> TTTTTTTTTGCAATAAAGCCTCAGAGAATTAGCAAAATTAATTTTTTTTT;> TTTTTTTTTAATCATACAGGCAAGGGCATTAACATCCAATATTTTTTTTT;> TTTTTTTTTCAATTCTACTAATAGTGCTGAAAAGGTGGCATTTTTTTTTT;> TTTTTTTTTCAGCTGTGGAGTAGATTAAGATGGCAGGTATGTTTTTTTTT;> TTTTTTTTTTGGGGGCACATGAGTGAGTTTTGGTACCAGGCTTTTTTTTT;> TTTTTTTTTACGAGTAGATTTAGAGTCAACATGTTCTGCGATTTTTTTTT;> TTTTTTTTTTCCCAATTTTAAATATCCATATAACAGTTGATTTTTTTTTT;> TTTTTTTTTCTAATTTTAAGACAAGATGATACAGTGTCTAGTTTTTTTTT;> TTTTTTTTTGCGGGCGCTAGGGCGCGAAGAAAGCGAAAGGATTTTTTTTT;> TTTTTTTTTCACCAGAACCCCAGCTGGCTTGTTGTGGAAGTTTTTTTTTT;> TGTCTAATGTATGGACAGTGGATAAACACGCGCCCTGTAGCGGCGCATTAAGCGCGGCGGGTGTGGTGGTTACGCGCAGCGTGACCGCTACACTTGCCAGCGCCCTAGCGCCCGCTCCTTTCGCTTTCTTCCCTTCCTTTCTCGCCACGTTCGCCGGCTTTCCCCGTCAAGCTCTAAATCGGGGGCTCCCTTTAGGGTTCCGATTTAGTGCTTTACGGCACCTCGACCCCAAAAAACTTGATTTGGGTGATGGTTCACGTAGTGGGCCATCGCCCTGATAGACGGTTTTTCGCCCTTTGACGTTGGAGTCCACGTTCTTTAATAGTGGACTCTTGTTCCAAACTGGAACAACACTCAACCCTATCTCGGGCTATTCTTTTGATTTATAAGGGATTTTGCCGATTTCGGGTAGAATTGGTAAAGAGAGTCGTGTAAAATATCGAGTTCGCACATCTTGTTGTCTGATTATTGATTTTTGGCGAAACCATTTGATCATATGACAAGATGTGTATCTACCTTAACTTAATGATTTTGATAAAAATCATTATAATGCCAGGGTCAGTGAGATGTAACACTACAGACCTCAGCTTCCTCTACTTTGCCTGGCATAGCCTACTGCACCATCCTTTTCAATGGAAGTAATTTGTCCCCCATGGGTTACACCCCCACCTAGACTACTTAAGAAGGTGCTATTGCTCCTGATTTCCAATGTTTGAATCTCCCTCCCACCATACCAGGCATAAAGGCTGTCACTCCCCAATACTAAGTGGCCCCAAGTTCACCACAATACAGCCAAGTGCATTGTTATCACATTCAGTCAAAGAATTTTCATTGGCAACAGTCCTCTCCAATCTGCCTATTCACTGTCCCTACATCAGGTGATAGTCCAGTTGTCAGACATGTGATCCCTGTTTGGGGACCCACAAGGCCTATCCAACCCATTGCTTTTAAAAGAGCTGGGGTTCTGGTGACTTCCACAACAAGCCCATCTGCTCTTAGTACAGCTTGTCTTAAAATTAGCTAGACACTGTATCATACCCCCTCCACTGCCCTATGATAAGGACAGCAGAGGGTTAGATTTACTTATCTGCACTCATGTGCCCCCAGCCTGGTACCAAAACTGATAATCTACTCCACAGCTGCATACCTGCCATCTTAGCCAAACCACACCAATCCAATTGCTGGGTCTCATATCATCTCTGAAGAAGTGATTACCTCATTACATGCTTGCTTGATATACCCACTTTCCTTATGAGGCACACCCATACTGAGGTAGCTATTTTACTATTGACTGGGTAAGCCAGTACAAAATAATCATAGGTGCACAGTCTGGACATGGGAACCCCTCTTCCTACTCACCTCTCTCAGAGGCAATGCCCCTTCATTAACCATGCACCCTAGGCCTTGGTACAAGTTGCCAACCTGCAGAGAACCAGTTAGCTGAAAGGCCAGGTTCTTCTTGATCTTGGTGCTTAGGGCAAACTTTTGGGATAGGCAAAAACAAGTCCTTTACACACCTCCAGTCTACAGTTCCATCAAAGTGGAACTTGGAATGTTATAAACTGCATCTATACTGTACTGCTAGTAGGCTTGTTTAATGCTTTCAACTCCTAGAGAATCACTTCAATCCTACCAACCAATAGTTCCCCATCACACAGATGGCTAAAGACCCTACCTCCCCTAAAGCCCTACTTCACACTGCAGGGACCTCCTAAGGGTCTTGGACCCTCCTCACTTGTTACTAGGCTATCATTCTACTGGTGCAGATACAGATTTTAGGTACCTGTCCTTGATGCACTTAGCTTTAACATGTCACATGCCAATGAAAATAGCAGCCACAGGGGGATATTCTAGGAGCAACATGGAGACTGTCTGCTACAACCACCAAACAGCTCATCCTCTGCATGAATACTTACTCTAGACCCCTGCATTCACCTTCCATGATTAATCACCAACTGAGTCTTGCAAAACCCAATTATGGTTATAGACAGACTGGCCCATGTTACCACTTAAACTCCATCTAGTCTGCAGTGTTCTGACCTATGCCTGAGGGTCCAGATAACCACTCTTCACTAAGCCCCCTGGAAGACAGTTAAGTCTATCTATCAGCCTCACATCCATCCCATTCTCTCTTTGAGATCTTATCAGGACTGATTGTATGTGAACAATATACTCCCAGGCTGGCCATTAGAGATTGGTTAGTGGTTGGCTGGACCAACACCCTTAAGCAACTAATAAGACCATGTGGGGTGTCCAGGCCTCATAAATCCTGAGCCTCTCAATCTTCCAGTGGCTCACCATTCCCATCCACACAACCTATTGGAACCATCAGAGTCATCACCTATATAGGGTGAAGTAGAGCTCCACCACCCCATAACTATACAGTGCACCTGGCCTCTGAGACTTGCTGTGATAACACAAACCCCAGGGCCAAATTGGGAAGATGCAATGACATTCCATTACTTCTCCAGGACAACATTTATTTGTTGCTGACTCCAGACTTAACAAGGAGTATTTGAGGCCACTGTTGGGGCCCTAACCCACCCAGCTCTTGACAGCTAATCTTAACCTCAAGGATTGACCATTGGGGGAGTCAACCAGCTTTGGCCCTGCTCAAGCAAACAATCCCCAGATGACCTGCTGGCAGGCACCCCTAGAAATATTGTGGGTTGCACTATTTCTTGCTCAGATGCTTCCCACTATAGCCCCACTCCAACTAGTACCACATCATTTTATGGATCAATCACAAAGGAGCCCCTATAGGCTGATTCTGTGTTTCAAAAAGTGAAGCCTATGTGCTCCATTGAGTCAGTAAATTAACACCACTAGAAGTTATCCAGCTAGTCAAGGGTTTTCCATATGTCCCAAGGTACTAGCTACAGCACTTGAATATGGTCTACTATGAGTGGGACTATTAATGTCATCTTTCTGTATAGCTGCCCCATTTAAAGCATATATGAAGTGCTAACATTGTGTTGGATCTTTATGCCACCAGATCCCCCTTACAGTATTCTCACCCAAATGGGATGAGAGTTGTATTAAGGCTAGTTAATCCCTAAGTCCATACATAGGACCACAGTAGCTTGGCTATGCTCACAATTTGCCATGTATATCAGTCCCAGAGGTATGCAAGACATTGCCCACATTTCAGAATGGTCCTGTCTTGTGGTTCCTTGCCTTTTGCACATTACCCTTGGCCTTCTACATAATGTGAGTCCTGGCTGCAATCTATGTATTGAAAGTAGGTAACCCTTCTCATTGTCAAGAACATCTGTTCCTAGCCACCCTGACCCTGCCTCCCTGAAGCTGCTCCCATAGGCCCACTGATCTCACTGCTTCTAATTGCATCCCTTGACTCTCTATCCCCTGAGAATTCCTGCTTGTGCAGCCTTGTGAGCCACTACCCAGTCAGGGTGTTAAGCCTTACCATGACCAGGTGCCCTCTATGACTAGCCCAAGACTCACAGACAGGATAGCCAGCTGTACCCCACACTCCTCTTGCCCTGGGCACTCTCATCAGTACCCTCAATAACCTAGCTGTCCACTCACTATCCTCAGACCAATTCTCCTTCTGCCAAAGGTCCAACATAGAGGACTCATCTGGGCTCAGGCAACTCAGGGCATATGGGACCATAGCTCAACTACAATAAAACCAGGGGCCACATAAGCTAGCAATCAGTGGGTGTAAGTGTCTGGGTGCATCAGCTGGTAAGACTGCCAGATTCTATGCAGGCCAATCATGAACCTACTAGTCCCTCATGGTCACTTTGTTCATCTAACAGATAGTTGCTTCAAACTCAAGACCTTACTAACCTTAGTCACTGGTTCTACCAGCCCAGGAATCCTCCTTGGGCTAGCCTCCAAGAAGCTTCAGACTCCTTAATACCAAGCAGCAGGAACAGTTTCAGCACCAAGAGGTGAGAACTGCTGTTAGCATCACTGACTTACAATCTCATGATAGCTAAGCATTCTTAGAACTCTTATATAACTCCCTATTACCAGAGACAGCCCTCAGGATTACTGATGGACCTTCTTCAAGTCTTTTCTAGCACAGGACCTACAGGGAGAGGGAAAGTCAGCTCCTATGGGGAATACAAGAGTTAGTCTTCAGTTTGTGGCTGAGGCTTCTTTGTGCTGGTTGCCTCTAAGACAAATTATTCTGGAATCTAATCAAGTTTACAAGGTCAGCATTATGACCCAGGTCAATAGCTTCTGGGAGGCTCTTCTAGTTTCCACCTTTGTACCAGTATCCTATTTAAGATAGGTCATGCATAGGGCTCTACACAATGAGTTCAGAGCCTTTGCAGCTTAAGGAAATCTCTCCTCCATAAAAGTTCTGCTTTGATGTCAATTCCCCTTGTACTTCCTGTGACTGCAACACAGTTGGACTGGTATTCCTCAACATCAACAATTAGTAAAAGCAATGGTTGTGACCAAGGAATGAGACCAGCAATTAATTGACATAGTTTAACTGTCAAACACTGAGAGATGGAGCCTGCAAGTGGGGCTTATCCCACAGAGTACTGTTTTCTGAGGAGCTGAGTTAACAGGTGGAGAAAATCCCAAAGATACTCTCCCAATGGCCAGTCCAAGCTTGAAGTCAATGCAACCTCTAGTAATAGGTAGAGGCTGCCACAAATGATGCCTACAAAGAGTAAACTTCTATATGTGGTAATGGCATCCAAGTAAAGGGCTAATGCAGAACAGAGCTTTTGTTAATGGGCAAGCTACTACTAAACCCTCTGGAGCATGTGTTAGTAGATACCTTCAACCTTGGAGCTCACTCAGAAAAAGCCTGAACCCAGAATTAAAACATCCTGGTGTACTCTGGCACCAGTGACACCATGGCTTTTTCAGGCCCCTGTGCCTGTTGCATGCAAACCTAAGAGTCTAAAGGTAATCTGTCAGCCAGGAGAGTGGTCTCCATGCCTCAGTGTGTAGGTGGGCAGTCATTCCTATACCATATAAAATGGAGTACATCTACAAGCACTGGACTACCTAGGTTTCCTGGATAGTAACTCTAACCAGACACACATGGCCTGGAGTGGAGTTACCCAACAGAACCCTGTCATATTTCCTAATCCACTAAAGTCTGTTACATACAGGCAGTTTTTGCTCTCTGCTGCCTGCCCAGCAGCTATGGTGATCAACTGGCTAGAATGACTTGTGTACCTACCCTAATTTTAATTTCACTCTGACATGCAGTTCAACAGGCTACCCCTTTTTATTGGTGGCTACATTTGGCTTAATTCTAACTGGTCAGAGATAAAGCTCAGCAGTGATATGAGCCCTTAGGAAAATTCCAGAGCACACACTAGCAGATGTTTTATCATGGAATATTATCAATGTAGCTCTGGGGGTAACTTTGAAAAGCTGTTCACTTACCTTTCCAGGGATAACTTGCATTTAGACATACTAGATTATCTTACATTCTGATATCACTAGTGTCCTGAAACAGGGCTTCATCATAATCCTTGTCACCTGTTAAACCTTTTATATGCCCTTGCTAGGGCCCAACTCTGTCTCCTGTAAAGTTAAAGTGCCTTCAGGAAGTTGGTGAGTAGACCTGAATAATTCATACTTTATCTCCTACACCAGGATGACTCAGTAGGACATCTCAGTCTCTAATACTCATACAAATACACTCTATTAGGGGCTGGGACACCTGATCCAGAAACAAAGTTTCTTAAGTACCTCTGTACAATTGAAGATAATGGTACTCAATGATATTTTGTGATTCAAATTTACAGAGAGCAGTAATGTTCCCAGTTTATCCTTAGATAGAGCAAAAGATTAAAGAACCTGGTTAATATTTAGGATCTGATGATCCTGCACACTTCTGAATGCCTTGAAATTCTTGTCCATTCAATACCCTGGTCTTAGGCCATATCCTGTTCTAGAACACTTATGCACAATCAATATGCATGGGCTGTGTGAGGGCTGCTATCTGTAGGCACTAATGGATTTGTAAGCTGGCTCTGTTTCTCTTACTTTCAGTATACCTATCAAGGTTTTGGTGTTGAAACCTGACTGACCACTGGCAAAGGGTGGGAAACTTAGGTTCCCTAGTATGCTAGCTTAGCAACCATAAGGTCTATTGTCTCAAATCAAAATCTAGGGGAACATGATCTGGATGCCCATATTCAAGCCAACAAATCTTGAACTGGGATTCCAAGGGCCTAACAACTATTCCACTTGGCACTTTAGCAGGCTCATTCATGCTCTGATCAGTTGCAATTTATGAAACTGTAGTCTCAGGTCCTAGGAATTATAGGTTGTACACTGGGCCTCCTGGGAATTGTTTGCTACTTGACCTCTTTCATGTACATGTTGATGGGGTAGTACTAATTAAGAGCCATAGTCATAAGTAGTTGGGCATGCTGAATCATCCAGTAGAAGGCTCCAGCATGAGGTGGCATTGATGAACAGCCTAAGCTTATTGCAAGCATGGCACATAGCACCTAACTTCATGACTGTTATTCATTTACCTGAGTATAGGATTTCATATAGATCCAAATAGGAACTAAGGTTCATAGTAGCCATCATGTTCAAAGCTATAACAAACATTAAATATATCCATGTCCTAAATGCATTAGGTGAACCAAGTCACAGGTACAGAAAGGGGATGCAGCACAAAAATTGATACTTGTAGAAAGAGGATTCAGATATATTGAGCTGTGCTACCATTAATAAAGATGGGTCCCATGAAGAGCATCTTCTGTTGTTAGGTCTGACTATGGCAGCAAATCCAGGTAAGGCAAGGACTAGTTCTCAAGTGACCTTTAAGTTGACTTTTAGCCTGTATTTCAAGGCTTAGAGGGCACAACTGTGTCTATAAATTGCCTAATGAATCCATAGACTTTACCAATGCTGTCTAGATATGCTTAAAGGAAGAGTGTTGTAGTGTATGAACTTTCTATTTGCTGCTGAGATATTAGTTGTGGATCCTAGTTGAATTTCTAAGTTAGGCAGGTATCTGGCTTGCAGGATCCATTTCTGCAAAGTAAGAGGGGGTCATTGCAGACCCATGCTATGTCTGTGAAAGATCTGTGCATATCTAGAGGTTAGGACTTCAGCTACCTGGGTTTGCATAAGAATAAGCAGACTAAAAGGCATGACAGAAGACTTCTTATGGGTAGCAGTCTTATTTTTAGAGTTCTTGGGAGATCAGATCTAAGGAGATTCACAAGAAACTAGAGTAGCATTGGAGATGAGTAACATATACACATATTACTACATGGTTTACTGCCTTAAATGTGGCCTAGGGTATTATGCTGGAGAGCTAGGTGTCAGTTCTAAAAAGGATAAGTCATGGGGGCCTTTCACAGCAAGTTACAAACTATGTTTAGTATCAGAACTTATTAAACATAACAGTAACCAAAGCCATGGTATGATGTACTATCTTTTTGTAGCACTAGGATACTATATTAACTACTCTTTAGTTTTGTCATGAGAAGTACACCTTATAGCATAGATTGAATGGGTGGATGTCTCTGTGGAGGTGTGTGCTTGGATTAGATGGTGTGAATAGAAAACTAAATACTGGATTGGACAAGTGTT;> TTAAGCTCTAAGCCATCCGCAAAAATGACCTCTTATCAAAAGGAGCAATTAAAGGTACTCTCTAATCCTGACCTGTTGGAGTTTGCTTCCGGTCTGGTTCGCTTTGAAGCTCGAATTAAAACGCGATATTTGAAGTCTTTCGGGCTTCCTCTTAATCTTTTTGATGCAATCCGCTTTGCTTCTGACTATAATAGTCAGGGTAAAGACCTGATTTTTGATTTATGGTCATTCTCGTTTTCTGAACTGTTTAAAGCATTTGAGGGGGATTCAATGAATATTTATGACGATTCCGCAGTATTGGACGCTATCCAGTCTAAACATTTTACTATTACCCCCTCTGGCAAAACTTCTTTTGCAAAAGCCTCTCGCTATTTTGGTTTTTATCGTCGTCTGGTAAACGAGGGTTATGATAGTGTTGCTCTTACTATGCCTCGTAATTCCTTTTGGCGTTATGTATCTGCATTAGTTGAATGTGGTATTCCTAAATCTCAACTGATGAATCTTTCTACCTGTAATAATGTTGTTCCGTTAGTTCGTTTTATTAACGTAGATTTTTCTTCCCAACGTCCTGACTGGTATAATGAGCCAGTTCTTAAAATCGCATAAGGTAATTCACAATGATTAAAGTTGAAATTAAACCATCTCAAGCCCAATTTACTACTCGTTCTGGTGTTTCTCGTCAGGGCAAGCCTTATTCACTGAATGAGCAGCTTTGTTACGTTGATTTGGGTAATGAATATCCGGTTCTTGTCAAGATTACTCTTGATGAAGGTCAGCCAGCCTATGCGCCTGGTCTGTACACCGTTCATCTGTCCTCTTTCAAAGTTGGTCAGTTCGGTTCCCTTATGATTGACCGTCTGCGCCTCGTTCCGGCTAAGTAACATGGAGCAGGTCGCGGATTTCGACACAATTTATCAGGCGATGATACAAATCTCCGTTGTACTTTGTTTCGCGCTTGGTATAATCGCTGGGGGTCAAAGATGAGTGTTTTAGTGTATTCTTTTGCCTCTTTCGTTTTAGGTTGGTGCCTTCGTAGTGGCATTACGTATTTTACCCGTTTAATGGAAACTTCCTCATGAAAAAGTCTTTAGTCCTCAAAGCCTCTGTAGCCGTTGCTACCCTCGTTCCGATGCTGTCTTTCGCTGCTGAGGGTGACGATCCCGCAAAAGCGGCCTTTAACTCCCTGCAAGCCTCAGCGACCGAATATATCGGTTATGCGTGGGCGATGGTTGTTGTCATTGTCGGCGCAACTATCGGTATCAAGCTGTTTAAGAAATTCACCTCGAAAGCAAGCTGATAAACCGATACAATTAAAGGCTCCTTTTGGAGCCTTTTTTTTGGAGATTTTCAACGTGAAAAAATTATTATTCGCAATTCCTTTAGTTGTTCCTTTCTATTCTCACTCCGCTGAAACTGTTGAAAGTTGTTTAGCAAAATCCCATACAGAAAATTCATTTACTAACGTCTGGAAAGACGACAAAACTTTAGATCGTTACGCTAACTATGAGGGCTGTCTGTGGAATGCTACAGGCGTTGTAGTTTGTACTGGTGACGAAACTCAGTGTTACGGTACATGGGTTCCTATTGGGCTTGCTATCCCTGAAAATGAGGGTGGTGGCTCTGAGGGTGGCGGTTCTGAGGGTGGCGGTTCTGAGGGTGGCGGTACTAAACCTCCTGAGTACGGTGATACACCTATTCCGGGCTATACTTATATCAACCCTCTCGACGGCACTTATCCGCCTGGTACTGAGCAAAACCCCGCTAATCCTAATCCTTCTCTTGAGGAGTCTCAGCCTCTTAATACTTTCATGTTTCAGAATAATAGGTTCCGAAATAGGCAGGGGGCATTAACTGTTTATACGGGCACTGTTACTCAAGGCACTGACCCCGTTAAAACTTATTACCAGTACACTCCTGTATCATCAAAAGCCATGTATGACGCTTACTGGAACGGTAAATTCAGAGACTGCGCTTTCCATTCTGGCTTTAATGAGGATTTATTTGTTTGTGAATATCAAGGCCAATCGTCTGACCTGCCTCAACCTCCTGTCAATGCTGGCGGCGGCTCTGGTGGTGGTTCTGGTGGCGGCTCTGAGGGTGGTGGCTCTGAGGGTGGCGGTTCTGAGGGTGGCGGCTCTGAGGGAGGCGGTTCCGGTGGTGGCTCTGGTTCCGGTGATTTTGATTATGAAAAGATGGCAAACGCTAATAAGGGGGCTATGACCGAAAATGCCGATGAAAACGCGCTACAGTCTGACGCTAAAGGCAAACTTGATTCTGTCGCTACTGATTACGGTGCTGCTATCGATGGTTTCATTGGTGACGTTTCCGGCCTTGCTAATGGTAATGGTGCTACTGGTGATTTTGCTGGCTCTAATTCCCAAATGGCTCAAGTCGGTGACGGTGATAATTCACCTTTAATGAATAATTTCCGTCAATATTTACCTTCCCTCCCTCAATCGGTTGAATGTCGCCCTTTTGTCTTTGGCGCTGGTAAACCATATGAATTTTCTATTGATTGTGACAAAATAAACTTATTCCGTGGTGTCTTTGCGTTTCTTTTATATGTTGCCACCTTTATGTATGTATTTTCTACGTTTGCTAACATACTGCGTAATAAGGAGTCTTAATCATGCCAGTTCTTTTGGGTATTCCGTTATTATTGCGTTTCCTCGGTTTCCTTCTGGTAACTTTGTTCGGCTATCTGCTTACTTTTCTTAAAAAGGGCTTCGGTAAGATAGCTATTGCTATTTCATTGTTTCTTGCTCTTATTATTGGGCTTAACTCAATTCTTGTGGGTTATCTCTCTGATATTAGCGCTCAATTACCCTCTGACTTTGTTCAGGGTGTTCAGTTAATTCTCCCGTCTAATGCGCTTCCCTGTTTTTATGTTATTCTCTCTGTAAAGGCTGCTATTTTCATTTTTGACGTTAAACAAAAAATCGTTTCTTATTTGGATTGGGATAAATAATATGGCTGTTTATTTTGTAACTGGCAAATTAGGCTCTGGAAAGACGCTCGTTAGCGTTGGTAAGATTCAGGATAAAATTGTAGCTGGGTGCAAAATAGCAACTAATCTTGATTTAAGGCTTCAAAACCTCCCGCAAGTCGGGAGGTTCGCTAAAACGCCTCGCGTTCTTAGAATACCGGATAAGCCTTCTATATCTGATTTGCTTGCTATTGGGCGCGGTAATGATTCCTACGATGAAAATAAAAACGGCTTGCTTGTTCTCGATGAGTGCGGTACTTGGTTTAATACCCGTTCTTGGAATGATAAGGAAAGACAGCCGATTATTGATTGGTTTCTACATGCTCGTAAATTAGGATGGGATATTATTTTTCTTGTTCAGGACTTATCTATTGTTGATAAACAGGCGCGTTCTGCATTAGCTGAACATGTTGTTTATTGTCGTCGTCTGGACAGAATTACTTTACCTTTTGTCGGTACTTTATATTCTCTTATTACTGGCTCGAAAATGCCTCTGCCTAAATTACATGTTGGCGTTGTTAAATATGGCGATTCTCAATTAAGCCCTACTGTTGAGCGTTGGCTTTATACTGGTAAGAATTTGTATAACGCATATGATACTAAACAGGCTTTTTCTAGTAATTATGATTCCGGTGTTTATTCTTATTTAACGCCTTATTTATCACACGGTCGGTATTTCAAACCATTAAATTTAGGTCAGAAGATGAAATTAACTAAAATATATTTGAAAAAGTTTTCTCGCGTTCTTTGTCTTGCGATTGGATTTGCATCAGCATTTACATATAGTTATATAACCCAACCTAAGCCGGAGGTTAAAAAGGTAGTCTCTCAGACCTATGATTTTGATAAATTCACTATTGACTCTTCTCAGCGTCTTAATCTAAGCTATCGCTATGTTTTCAAGGATTCTAAGGGAAAATTAATTAATAGCGACGATTTACAGAAGCAAGGTTATTCACTCACATATATTGATTTATGTACTGTTTCCATTAAAAAAGGTAATTCAAATGAAATTGTTAAATGTAATTAATTTTGTTTTCTTGATGTTTGTTTCATCATCTTCTTTTGCTCAGGTAATTGAAATGAATAATTCGCCTCTGCGCGATTTTGTAACTTGGTATTCAAAGCAATCAGGCGAATCCGTTATTGTTTCTCCCGATGTAAAAGGTACTGTTACTGTATATTCATCTGACGTTAAACCTGAAAATCTACGCAATTTCTTTATTTCTGTTTTACGTGCAAATAATTTTGATATGGTAGGTTCTAACCCTTCCATTATTCAGAAGTATAATCCAAACAATCAGGATTATATTGATGAATTGCCATCATCTGATAATCAGGAATATGATGATAATTCCGCTCCTTCTGGTGGTTTCTTTGTTCCGCAAAATGATAATGTTACTCAAACTTTTAAAATTAATAACGTTCGGGCAAAGGATTTAATACGAGTTGTCGAATTGTTTGTAAAGTCTAATACTTCTAAATCCTCAAATGTATTATCTATTGACGGCTCTAATCTATTAGTTGTTAGTGCTCCTAAAGATATTTTAGATAACCTTCCTCAATTCCTTTCAACTGTTGATTTGCCAACTGACCAGATATTGATTGAGGGTTTGATATTTGAGGTTCAGCAAGGTGATGCTTTAGATTTTTCATTTGCTGCTGGCTCTCAGCGTGGCACTGTTGCAGGCGGTGTTAATACTGACCGCCTCACCTCTGTTTTATCTTCTGCTGGTGGTTCGTTCGGTATTTTTAATGGCGATGTTTTAGGGCTATCAGTTCGCGCATTAAAGACTAATAGCCATTCAAAAATATTGTCTGTGCCACGTATTCTTACGCTTTCAGGTCAGAAGGGTTCTATCTCTGTTGGCCAGAATGTCCCTTTTATTACTGGTCGTGTGACTGGTGAATCTGCCAATGTAAATAATCCATTTCAGACGATTGAGCGTCAAAATGTAGGTATTTCCATGAGCGTTTTTCCTGTTGCAATGGCTGGCGGTAATATTGTTCTGGATATTACCAGCAAGGCCGATAGTTTGAGTTCTTCTACTCAGGCAAGTGATGTTATTACTAATCAAAGAAGTATTGCTACAACGGTTAATTTGCGTGATGGACAGACTCTTTTACTCGGTGGCCTCACTGATTATAAAAACACTTCTCAGGATTCTGGCGTACCGTTCCTGTCTAAAATCCCTTTAATCGGCCTCCTGTTTAGCTCCCGCTCTGATTCTAACGAGGAAAGCACGTTATACGTGCTCGTCAAAGCAACCATAGTACGCGCCCTGTAGCGGCGCATTAAGCGCGGCGGGTGTGGTGGTTACGCGCAGCGTGACCGCTACACTTGCCAGCGCCCTAGCGCCCGCTCCTTTCGCTTTCTTCCCTTCCTTTCTCGCCACGTTCGCCGGCTTTCCCCGTCAAGCTCTAAATCGGGGGCTCCCTTTAGGGTTCCGATTTAGTGCTTTACGGCACCTCGACCCCAAAAAACTTGATTTGGGTGATGGTTCACGTAGTGGGCCATCGCCCTGATAGACGGTTTTTCGCCCTTTGACGTTGGAGTCCACGTTCTTTAATAGTGGACTCTTGTTCCAAACTGGAACAACACTCAACCCTATCTCGGGCTATTCTTTTGATTTATAAGGGATTTTGCCGATTTCGGAACCACCATCAAACAGGATTTTCGCCTGCTGGGGCAAACCAGCGTGGACCGCTTGCTGCAACTCTCTCAGGGCCAGGCGGTGAAGGGCAATCAGCTGTTGCCCGTCTCACTGGTGAAAAGAAAAACCACCCTGGCGCCCAATACGCAAACCGCCTCTCCCCGCGCGTTGGCCGATTCATTAATGCAGCTGGCACGACAGGTTTCCCGACTGGAAAGCGGGCAGTGAGCGCAACGCAATTAATGTGAGTTAGCTCACTCATTAGGCACCCCAGGCTTTACACTTTATGCTTCCGGCTCGTATGTTGTGTGGAATTGTGAGCGGATAACAATTTCACACAGGAAACAGCTATGACCATGATTACGAATTCGAGCTCGGTACCCGGGGATCCTCCGTCTTTATCGAGGTAACAAGCACCACGTAGCTTAAGCCCTGTTTACTCATTACACCAACCAGGAGGTCAGAGTTCGGAGAAATGATTTATGTGAAATGCGTCAGCCGATTCAAGGCCCCTATATTCGTGCCCACCGACGAGTTGCTTACAGATGGCAGGGCCGCACTGTCGGTATCATAGAGTCACTCCAGGGCGAGCGTAAATAGATTAGAAGCGGGGTTATTTTGGCGGGACATTGTCATAAGGTTGACAATTCAGCACTAAGGACACTTAAGTCGTGCGCATGAATTCACAACCACTTAGAAGAACATCCACCCTGGCTTCTCCTGAGAAAGCTTGGCACTGGCCGTCGTTTTACAACGTCGTGACTGGGAAAACCCTGGCGTTACCCAACTTAATCGCCTTGCAGCACATCCCCCTTTCGCCAGCTGGCGTAATAGCGAAGAGGCCCGCACCGATCGCCCTTCCCAACAGTTGCGCAGCCTGAATGGCGAATGGCGCTTTGCCTGGTTTCCGGCACCAGAAGCGGTGCCGGAAAGCTGGCTGGAGTGCGATCTTCCTGAGGCCGATACTGTCGTCGTCCCCTCAAACTGGCAGATGCACGGTTACGATGCGCCCATCTACACCAACGTGACCTATCCCATTACGGTCAATCCGCCGTTTGTTCCCACGGAGAATCCGACGGGTTGTTACTCGCTCACATTTAATGTTGATGAAAGCTGGCTACAGGAAGGCCAGACGCGAATTATTTTTGATGGCGTTCCTATTGGTTAAAAAATGAGCTGATTTAACAAAAATTTAATGCGAATTTTAACAAAATATTAACGTTTACAATTTAAATATTTGCTTATACAATCTTCCTGTTTTTGGGGCTTTTCTGATTATCAACCGGGGTACATATGATTGACATGCTAGTTTTACGATTACCGTTCATCGATTCTCTTGTTTGCTCCAGACTCTCAGGCAATGACCTGATAGCCTTTGTAGATCTCTCAAAAATAGCTACCCTCTCCGGCATTAATTTATCAGCTAGAACGGTTGAATATCATATTGATGGTGATTTGACTGTCTCCGGCCTTTCTCACCCTTTTGAATCTTTACCTACACATTACTCAGGCATTGCATTTAAAATATATGAGGGTTCTAAAAATTTTTATCCTTGCGTTGAAATAAAGGCTTCTCCCGCAAAAGTATTACAGGGTCATAATGTTTTTGGTACAACCGATTTAGCTTTATGCTCTGAGGCTTTATTGCTTAATTTTGCTAATTCTTTGCCTTGCCTGTATGATTTATTGGATGTTAATGCTACTACTATTAGTAGAATTGATGCCACCTTTTCAGCTCGCGCCCCAAATGAAAATATAGCTAAACAGGTTATTGACCATTTGCGAAATGTATCTAATGGTCAAACTAAATCTACTCGTTCGCAGAATTGGGAATCAACTGTTATATGGAATGAAACTTCCAGACACCGTACTTTAGTTGCATATTTAAAACATGTTGAGCTACAGCATTATATTCAGCAAT;> TTTTTTTTTTGAGTGTTGTTCCAGTTAGCCCGAGATAGGGTTTTTTTTTT;> TTTTTTTTTGGGAAGAAAGCGAAAGCGTGGCGAGAAAGGAATTTTTTTTT;> TTTTTTTTTAAGTGTTTTTATAATCACGCCAGAATCCTGAGTTTTTTTTT;> TTTTTTTTTAATGGATTATTTACATACGCTCAATCGTCTGATTTTTTTTT;> TTTTTTTTTAATTTACTGACTCAATAACTTCTAGTGGTGTTTTTTTTTTT;> TTTTTTTTTCACAGAATCAGCCTGAGCTTCACTTTTTGAAATTTTTTTTT;> TTTTTTTTTGTGATTGATCCATATAGTATAGGGGCTCCTTTTTTTTTTTT;> TTTTTTTTTTAGTTGGAGTGGGGCAATAAATGATGTGGTACTTTTTTTTT;> TTTTTTTTTATCTGAGCAAGAAATTCTCTATAGTGGGAAGCTTTTTTTTT;> TTTTTTTTTATATTTCTAGGGGTGCGGTAGTGCAACCCACATTTTTTTTT;> TTTTTTTTTGATTGTTTGCTTGAGCCAGCAGGTCATCTGGGTTTTTTTTT;> TTTTTTTTTCCCCCAATGGTCAATCCCAAAGCTGGTTGACTTTTTTTTTT;> TTTTTTTTTTCAAGAGCTGGGTGGGAGGTTAAGATTAGCTGTTTTTTTTT;> TTTTTTTTTTCAAATACTCCTTGTTGGCCCCAACAGTGGCCTTTTTTTTT;> TTTTTTTTTGCCTTGAATCGGCTGAGGGCACGAATATAGGGTTTTTTTTT;> TTTTTTTTTTCTGTAAGCAACTCGTCAGTGCGGCCCTGCCATTTTTTTTT;> TTTTTTTTTGAGTGACTCTATGATAATTTACGCTCGCCCTGTTTTTTTTT;> TTTTTTTTTAATAACCCCGCTTCTAGACAATGTCCCGCCAATTTTTTTTT;> TTTTTTTTTTGCTGAATTGTCAACCATTTAAGTGTCCTTAGTTTTTTTTT;> TTTTTTTTTTTCATGCGCACGACAAATTAAGTGGTTGTGAATTTTTTTTT;> TTTTTTTTTGGTGGATGTTCTTCTTAATCAGGAGAAGCCAGTTTTTTTTT;> TTTTTTTTTAGTGCCAAGCTTTCGGTAGTAAAACGACGGCCTTTTTTTTT;> TTTTTTTTTCCAGTCACGACGTTGCCAACGCCAGGGTTTTCTTTTTTTTT;> TTTTTTTTTCAACCACTAACCAAACCTGGTGTTGGTCCAGCTTTTTTTTT;> TTTTTTTTTCCTGGGAGTATATTCATATCTCTAATGGCCAGTTTTTTTTT;> TTTTTTTTTAGTCCTGATAAGATTCCAGTTCACATACAATCTTTTTTTTT;> TTTTTTTTTGGGATGGATGTGAGGCTCCTCAAAGAGAGAATTTTTTTTTT;> TTTTTTTTTCTTCCAGGGGGCTTAGAGATAGACTTAACTGTTTTTTTTTT;> TTTTTTTTTCCTCAGGCATAGGTCAGAGTGGTTATCTGGACTTTTTTTTT;> TTTTTTTTTAGTTTAAGTGGTAACAACTGCAGACTAGATGGTTTTTTTTT;> TTTTTTTTTCATAATTGGGTTTTGCCCAGTCTGTCTATAACTTTTTTTTT;> TTTTTTTTTAGGTGAATGCAGGGGCGGTGATTAATCATGGATTTTTTTTT;> TTTTTTTTTTTCATGCAGAGGATATAAGTCTAGAGTAAGTATTTTTTTTT;> TTTTTTTTTTTGTAGCAGACAGTCAATGAGCTGTTTGGTGGTTTTTTTTT;> TTTTTTTTTTAGAATATCCCCCTGTCCCTCCATGTTGCTCCTTTTTTTTT;> TTTTTTTTTTGTGACATGTTAAAGCGCTATTTTCATTGGCATTTTTTTTT;> TTTTTTTTTACCTAAAATCTGTATCTGCATCAAGGACAGGTTTTTTTTTT;> TTTTTTTTTCTAGTAACAAGTGAGGCCAGTAGAATGATAGCTTTTTTTTT;> TTTTTTTTTAAAGCCCCAAAAACAGCCGGTTGATAATCAGATTTTTTTTT;> TTTTTTTTTGCATGTCAATCATATGGGTAATCGTAAAACTATTTTTTTTT;> TTTTTTTTTAAACAAGAGAATCGATCCTGAGAGTCTGGAGCTTTTTTTTT;> TTTTTTTTTCAAAGGCTATCAGGTCTTTTTTGAGAGATCTATTTTTTTTT;> TTTTTTTTTGAGAGGGTAGCTATGCAAATAAATTAATGCCGTTTTTTTTT;> TTTTTTTTTAACCGTTCTAGCTGGAAATCAATATGATATTCTTTTTTTTT;> TTTTTTTTTCAGTCAAATCACCAAATGAGAAAGGCCGGAGATTTTTTTTT;> TTTTTTTTTGCCTATCCCAAAAGAACCAAGGACTTGTTTTTTTTTTTTTT;> TTTTTTTTTCAAGATCAAGAAGACCTTTTTGCCCTAAGCACTTTTTTTTT;> TTTTTTTTTCTAACTGGTTCTCTGCGCACCTGGCCTTTCAGTTTTTTTTT;> TTTTTTTTTTGTAATACCCTGACTAGGAAACATTATGACCCTTTTTTTTT;> TTTTTTTTTATCGGTTGTACCAATAACGAGCATAAAGCTAATTTTTTTTT;> TTTTTTTTTATTGTTATCCGCTCACAACAATTCGAATCAATA;> AAAGAAATACATGGCTTTTTTGTATTTGGAGTTGGGTAGCCA;> GGGTCAGAAGGAGCAAGTTTGCAAGGAAGAGCATAAATATCT;> GTTTGAGGCAATTCCAACTCGTCATTAGACTTTACCGATTGG;> GAGAGTCAAGGGATGGGAGCAATTCCTGCCCGAACCATTCTG;> AAGAAATGGTAATATCCAGTAACTGAGAACTTTAAGCCACCA;> TTTTTTTTTGGAGGATCCCCGAACCAATAGGAATTTTTTTTT;> CGCGCAGACACCTATTATTCTGAAACTTTTAAGTTACAAAAT;> TTTTTTTTTACGTGGTGCTTGAAATTTTTGTTATTTTTTTTT;> GAGGATATATCCTGTATTAACAATATCACGGGGAAGCACTAA;> TTTTTTTTTCTTGTGGGTCCCCAAAAATGGGTTGGATAGGCTTTTTTTTT;> TTTTTTTTTACTGGACTATCACCTGGATCACATGTCTGACATTTTTTTTT;> TTTTTTTTTCAGATTGGAGAGGAGGAGGGACAGTGAATAGGTTTTTTTTT;> TTTTTTTTTATGGTGGGAGGGAGATAGCCTTTATGCCTGGTTTTTTTTTT;> TTTTTTTTTAATTCTTTGACTGAATTGCTGTTGCCAATGAATTTTTTTTT;> CACCACACCCGCCGAGCACTAACTCCAGGAAACCTGCAAATAAGCATAT;> CGCCAGCTCTGGCCAGCCCTAGGTGAGGTCCCACTCATAGTAATGTTAG;> CTGATATAACTAATACCCTCATATATGCTTAATAGCGGTCAGTATTAAC;> TACATCGGGAGAAATTTGCACCAGTGCCCGCAGTCATCCTGGACTCACC;> AATTCAATTACCTGGTCGCTATTAATCTGACCTCCTGGTTTTTTTTTTT;> AAACACCGGAAGAGTTCTAAGAATGCATCTTCCCAATTTGTTTTTTTTT;> TGTAAGGTTGACCTACTTTTAACAGGGGAATTGACAAGCTTAGGCTGTT;> GGGTCATCATGCTGTCCTAGGACCTGCTGGAATAATTTGTCTGGGCTGT;> CTGCAAAGGCTCTGCAAAGGTCTTATGAGTAGCAACCAAAAGGAAAGGA;> GCCAGTTACAAAATGTTTTGACTGATAACACCAACCGAGAGGCTTTTAA;> TAACATAAAAACAGGTAATTGAGGACAGATCTTGATACCACAACATAGC;> TTTTTTTTTCAAAGCGCCATTCGCCAAGCAATAGCTAGCAAACGTAGTG;> TTATTTTAAATTATAGAGTGAGGGGTAGGCAAGGCATCGGCAAACAGCT;> TTTTTTTTTGGCGCATCGTAACCAATCACCAGTAGCCGGATAGGTCACG;> TTTTTTTTTTGTTAAAATTCGCAATGAAAGTATTACGCCACCCTCAGAA;> CGTAACAAACTATACCAAGGAGGATTCCAACAGCAACAATAGAGTTGTT;> TCTTTCCAGACGCCGAACCACCCTCATTGAACGCGAGAAAGTCGTAGCT;> AGCATGAATGAGCCCATACTAGGGAAGTGCTTAGCTATCATGTAAGGTT;> CAACCATCTACAGAAGTTTGGATCTATAATGCTTTAAACATACAGCAAA;> TTTGTTATAAAACAGCGAAACCCTCTTTCTTGGATCATTAGACGGGAGA;> ATTTCAAAATCTACAATAAGTGTGTCTGTCGAGGTGATGGCCCACTACG;> AGACTGCGTAAGAGCAACACTTTAGGAACAAGAACCTAGACAAGGGGCC;> TTTTTTTTTCAAGCATGTAATCTCCACTTTGATGGAACTGTTTTTTTTT;> AGAAGTTTTGCCAGCCCTCAATGAAATCGAGGGTAGGCTGTCTGTGTAG;> TTTTTTTTTCAGAGATGATATCATACAGTATAGATGCAGTTTTTTTTTT;> AAGAGTCCACTATTATCGGAAATTAGAGAGCGTCACCACCAGGGTGGCT;> TATTGGGCATTGTGAATTACCAGTCAGGTCAATAGTAACTCCAATCGGA;> GTTTGATCAAAGGGACCCTAAGCGTAACGCGGGAGAACCGTT;> GTCCACGAGTATGTTATCTTAGGAGAAACAATGAAATTCAGT;> TTTTTTTTTTGGCCCTGAGAGAGTTGCAGCAAGCGTGAACCA;> CGAAAAACCGTCTACAGGCGAGATTAAGAAGAAAATGAAAAA;> CGGCGAAGAGCGGGGAACGGTAGTGAGGCATTTTGTGGCAGA;> TTTTTTTTTGGGCAACAGCTGATCAAATCAAGTTTGCGCGTA;> GATTAAAAGTCTGTAAACGCTGACCAGTAAAATACCGAACCC;> GGAGGCCAGCGGTCACGCTGCAGGGAGCAGGGTTCTTGTAGA;> GCTTTCCTTGATTATAATATCCCTTCTGGTCTTTAACCGCCT;> TTTGACGTGCCTGAGTAGACGTATTGGGCGCCATTTTTTTTT;> GTAGCAATACTTCTTCGTTAGTTGACGGGTCACAAACGTTGG;> TTTTTTTTTGGAGAGGCGGTTTGAGAACTCAAACTGAATACG;> TTTTTTTTTCTGCATTAATGAATCAGACAATATTTCTCAGTC;> CAGCAATGCAACAGTGCCACGTTGAATGTCATAGCCACCATT;> GGGGCAGACCTCAAATATCAAAGATTAGCACCACCCCAGCAT;> AGTTGGCCAACACAGACCATAGAAGATAAAACAGAAAACATC;> TTTTTTTTTTAATGAGTGAGCTAACTAGCATCACCAATACAT;> AGCCGTCGCATACCTCTGGGAAAATGTGCAGGTCTTGTAGGA;> GAAGTTTAATAGATTTGCTGACTAATGAAAAATCTTTATTAG;> TTTGCTACCAAGGGGTCCTATAAATTGAGGAAGGTCGCCACC;> GTCAGACCCAGAGCCACTTCAATCAATATCTGGTCTTAGGAG;> TACATTGAGTATGTTTAAGTTAATCAGACAACAAGAAAGAAT;> CGTTTTGTTTTCGGGCTATTAACCTGAAAGCGTAAATCGGCC;> CTCAGGACTAGTGATCTGCTAGTGTGGAGTAAGGGCTCATCC;> GCCACCCATAATCTATAATATAGTTTGCGCCATTAAATAAAA;> CAGAGCCGAACCACAGCCCGAGTGGACTCCAACGTCGAGGTG;> CAAAATCGGCAGGTCACATTAAATGTGAGCGAGTTTTTTTTT;> CCACCCTTTGTTCCAGTTTGGATATCAAATATGGTGGACAAA;> GCCGCCGGGAACCGCAAGTTAGTTACCCTGTAGCGAACTGAT;> AAATCCTAACAGTTAATGCTTGGATGGAAGGGTTAGCTTTGA;> TTTTTTTTTGGTGTAATGAGTACGTTAATATTTTTTTTTTTT;> TTTTTTAAGTTGAGCTAGTAGCTTTTTAACAACTATCTGTTA;> ATATATGTGAGTGAAAACATCGTATCACGAAGGATCTGGAAG;> ATAACCTCACCCACACCAGCTGTCAATAGTGAATTGCTGATG;> CTATGGTAAAACCTGGATATGGTATTCACATTTTTGCGGATG;> TTTTTTTTTACAAATAAATGTTCCAAGACCCTTTTTTTTTTT;> CAAATCCTGAAGCTTCTTGGAGTGCTGATCCCCTACCAGTTC;> TGGGCTGAGGTTGGAGACTACGTTCATGATTGGCCCCTGGTT;> GGCTAGCTGTAAATTATCAAAAATCTGGCAGTCTTTGATTGC;> TTTTTTTTTTGGAATGTCATTGTGAAGTAGGGCTTTTTTTTT;> TTTTTTTTTGCCCTGGGGTTTTCTTTAGCCATCTTTTTTTTT;> ATCCTGATAGAGGCCTATAATGAGCCTTCTTTCATCAATGCC;> TAGGTCCACTAACTAGGTCAACTATGGCCGATATATCGGAAC;> TTTTTTTTTTCTCAGAGGCCAATTGGTTGGTAGTTTTTTTTT;> AGCCTCACCAGGAGAGCATGCCTTGCAGCCTCAGCACAGTCA;> CTTGTATGGCAGAGGCATTTTCATGTTCACTGGTAAACTCAT;> GAGAATCGCCATATATACAGTAGGGCTTAACTGACTTTCCCT;> AAACTTGATTAGATTCCAGTGCACTGTATAGTTTTTTTTTTT;> TAAAGTAACAAAGAAAGGTCCTACTAGATAAGAATTGATGCT;> CGAGCCAACTGAAGTGTGCTATATCATATGTGATACCTCTTG;> CCTTAAGGGGTATTAGCCGTTGTTGATGGGCTCCATGCACCC;> TTTCCTTAGGAATCCAACCATACAGTTAAATCAAGCTAATTT;> TTTTTTTTTATGGGAATGGTGAGCCATCACAGGAAGTACATC;> ATCGAGAACAAGCAAAACCAATCGTCACGGAGTTACTAAACA;> TTTATTTTCATCGTATCATTCGACAGCATTCGGTCCTGTGAA;> TCCAACTGTGGGATCCAGCTCCTCAGAATTCTGTACCTGTAG;> TGCTTTTGAACATGCAGGTAATATTCATAGAACTGACACCTA;> TTGGTCAATTACCGCGCCCAAAATAATCGCAACGGCGCCCAC;> TCATTCCCCTTAGTTCCTATTACGAAGGATTGTGTACCCATC;> AGGCCCAGTACTCTGTGTTGCTGCATTTATGCTTGGAGGCAG;> AGCTACAACCAAGCCTCATCTCTAGTTTGATAGCGTCTAATA;> AACTCTGATCTTTGGGATTTTAAAAGCTCTGCATCAGGTCAC;> TAACGAGTGGACTGGCCATTGCCCTTTACTACAAGTTGCCTT;> CGTCTTTCCAGAGCATTAGTTAACGGAGGCAAAAGTAGATCT;> AGAAATGCATATTATTTATCCGAACCTCCGCGACCTACGTAA;> CATCATTTAGCAGCCTTTACAAGAGATACGAACTGTCATTAC;> TAATTCTGGGTTCACAGGCACGCATTGGCTAATATACTTTGC;> CATGCAAGGCTTTTTCAGAGGGGAAGCGGCCATTATCAAGCT;> GCCATGGTCCTTTAGAAAGTTGAACTAAGAAGAAACTTTAAT;> TGTCACTCCGAAGCCCTTTTTACTCCTTTATCCAGGCCATGT;> ATAACGGCCGAAATCGGCAAAAAAGAACTTAGAGCCAAGTGT;> ATTACGCCTGGTTTGCCCCAGTCAGGGCGCCGTAACGCTTAA;> ACATACATAAAGTATAAGGCTTGCTTTTGCGGGAGGGAAAAT;> TTTTTTTTTGGCACCGCTTCTAAGCCTTTATTTTTTTTTTTT;> TAGTGGATATGGTAAACTTAGGCAATTTTAAGGCTGGCTGAC;> TGTTGGGAAAATTCAGGGAAGTAGGTACAAATGTAATGAAAC;> TTGAGGGATATGGTTGGCTCAAGAAATGTTCACAGTTCAACT;> CCAGTTGCTGACCACCGTAATCAGTACCTTACTTCGGGGGTG;> GCATGTCTCATTAAATAACGTTGCGCCGCTACAGGTTTGGGG;> TTTTTTTTTTTGAGGGGACGACGCCGACTTGAGCCATTTGCT;> AGCAGCAGTTAGAAACAGGAACCATCACGCAAATTCTAAACA;> ACCATTACCTGTTGTTGCTGGGTAATAACATCACTAGCACGT;> TGTAGCGGTCACGCGAACGTGAATTTGAACGGGGTGTAAAAC;> AAGTTTTAGGAAGGTGGCAAGTTTCATTGCAACTACTGTAGC;> TCCCTTACGAAAAACCGTCTACCAAATCGATAAAGGCCAGAA;> TTGGAAATCAGGAGCACTTAGATTAGGGGTAAATAAATCAGA;> CTTGGCTTCTAGGTCATTGAAATACACAATGTAAGTCAGAAC;> GAGTGACTCAAACAAGGAAGCGGCATTAAAAGGTACCAGAGC;> TTTTTTTTTAGGAGGTCCCTGATCTAACCCTTTTTTTTT;> TTTTTTTTTCTACGTGAACCATCACTCAGGGCCGAAATC;> CACGACTTGACCCTTGAGGTCTGTAGTGTTTTTTTTTTT;> TTTTTTTTTAATTCTACCGATGGCCCATTTTTTTTT;> TACAGGACCATTATCATCAGAAGGCGGATAAGTAAAACGCCG;> GGAACATACAGTGCCCATATCGAAGCAGTGGATTATACTTCT;> TTTTTTTTTAATCAGCTCATTTTCCCCTGCCTATTTCGGATG;> CTATCTACTCAAGACGTACTCGCCCTCAAATCCATGCCCAAT;> TAAGTATTTTTGCTTTTATCCAACCACCACACCCGAGCTTGA;> GATAGCAAGGAGGTGAAGATGACTGATGAGAGAGGCGAATTA;> TTTTTTTTTAATATTTAAATTGTAACCGCCACCCTCAGAACA;> TGATAGGCAGTACACCGGCTTGTAGAACCAGTGACAGATTGT;> AAAGTAAGTGCATAGCTTAGATTGTCCAATCCAGTGCGCGTG;> GCTTACACACAGCCTATAATGAAGTACGGTTTAGACAAACAC;> AGTCAGGTGGGTCTTGAGTTTGAAGCCTAATTGCCAGTGGTC;> TCGTCACTATACTGTTATTGTATGGAAACAGTACAAATTACA;> 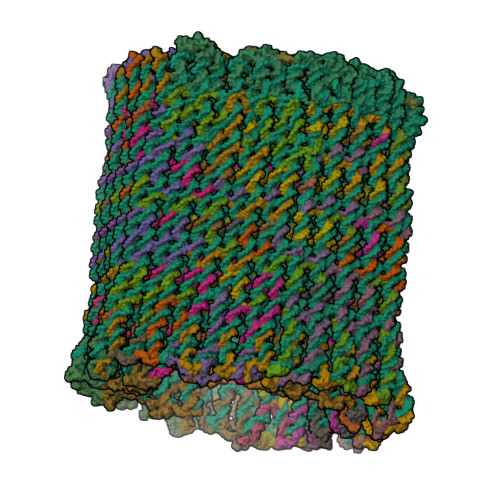AGGAACCGTTAGCGTTAGAGATGTACTTCTCTCCAACTTTGA;> CACCTAAGTTTCCCACCCTCTATCTAATCCAAGGATAGGGCA;> AAGCTAGTGCTAAAAAAAAGATAGTATCCACACACACCTCCA;> TTATGGGCATCCAGCTAAAGTATAGCAATAGTGCCACACTTA;> TGGAATCGATTTTGCCTCATACATGTACAGAGCCATAGCTTA;> CTGTATGGGATTACTATTAGTAAATGAATTTAGTTAATTTGA;> CAGAGGGGTGTAATAGGGAGTTATATAATTATTGCAACTGAT;> AAACAACAGCCAACGCTCACTCCCATCTTCTGACCTAAATTT;> ACAGTTTCATAATTTGGTTACTGTTAGCTACATCATACCATG;> ATGTGCCAGGACATCCGACTTGGTTCACGAACTCATCTCCAA;> CTATACTATGGCTAGAAAGAGATTTGTACACAGCTTAGAAGT;> CTTTTTCATGAGGAGGCTTTGTGTAGAAAATATCCCATCCTA;> TTTAATGTGAAGTTATACTGCAGCATAATACCCTATCTGATA;> TTTTGTGCTGTTCTAGTAGCTTGCCCATTGCTCCAAGTCAAC;> CGGATATACCAACTAACAACAATGGTAGTCATCGCAGCCTTA;> TTTTTTTTTCAACGCAAGGATAGAACCCTCATATTTTTTTTT;> TTATACCTTATGCGTTGGGGCCAATAGCAGGCTATAAAATCA;> CAAGCCAGTTAATGAAGGGACTTACCAGATATGACCCCCGAT;> CGTGACCCCCTCTTCTCAGCAAGGTAGTCTGGCATAAATCCT;> ATACATAATATGCACAGATCTGATCCTGACTAGGATGTACTC;> TCATCAGACAACATTATTACAATAAAACCATACACGAGTTAC;> TTTTTTTTTGGGTGTGCCTCATAAGGCTTATTCTTATGCAGC;> AGGCATATACCCATATCTCCTAATACACTAGCTTTACTAATT;> TTTAGTCTTGAGAAGGCTAAAGAGGGTTAAGGTATCTACTAA;> CTTCTGTCAAAAGGAATTACGAATGCAGCTTCATCTATGGAT;> AACCAAACCCTCGTTTACCAGGAAAGATCCAAATCACACTCT;> CGATAAACTCTTCAAGGGAACACCCACACCAGAGTACACCAG;> AATAGTAAAATGTTTCATAAAATGAATAAGCGAAACAAGAAC;> TGAATCCAGGGGGTGATCTCCCAAGAAGCTAAAACCTATGAA;> TAACTTGGCTGAGGCCAACTAGGAAACTACGACAATAAACAA;> TGACCATAAATCGAAGGTTCAGAAAACGAGCTTATCCTTTTT;> TTGCATCAAAAATTCACGTTGGTACAACAACCAGCCCGACAA;> AAGCGGATAGTTTGGCTCTCCGGAATCGTAGACTGCTTGTGA;> TATAGTCAAATATCACTAAAGTATAAGGGTACCTTTGCTGAA;> TTTTTTTTTTTCATTTGGGGCGCAAAAATCAGGTCGCTTCAA;> AATATAGGCCCGAAAGACTTCAGAAGCAAAAGGCTACAATTC;> TGACAAAGCGTTTTAATTCGATTTACCCTAATTGTATGAAAG;> ACCGGAAGCAAACAAAGATTTGCGGAGTTACAAATCTCCCTG;> CAGAGACGTGCTACGTGCCAAAATAATTTCATAATATCAGTA;> TCCTTTTCATTCAATCTATGCAGTAGTTAGGCCCTACAACTA;> CAGAGCCCTTTACACAAAAGGAGTAACATTATCAT;> CACCAGAAACTTCCACAGGACGTTATTAATTTTAA;> GGAGACATATGAGTCCCTAAAGGGAGGCCAGGAAC;> CCTTGTGAGGTTGAACCGGAAAGGCCATCTTTTCA;> ATAGAGTTCTGGATTTCAATATTGACAATGAGAAG;> CTGAGTCTCTGAATTCATCATGCTTCAGGGAGGCA;> TGTACAGAGGTACTTAATTCAGAAGTGTATAGAGG;> TTGAGTAGTGTACTTGCGTAGAGCAGGAATTCTCA;> CAGGTTCAGCGGGGAGCCCGGATTGATTGAGAAAC;> CAGTACCTCCTAAATCTGTGAATATACAGTAACAG;> TTTTTTTTTACATCTCACCTCTTTACCTTTTTTTTT;> GTGGACTCCAACGTGGTGGTTAATACCCGAACAAA;> AACAGAGATAGAACCAGAACAATAAAAAAATTAAA;> GCTGGATGGGACATATGGAAAACGAACCACCAGCA;> CTTGGAGCACATAGGAATACTCTCAGTTCCTGTTT;> TTCAAGTGCTGTAGGTGGCATTAAAACATATCAGA;> ACAGAAAGATGACATTTAAATTTTCAAATCCCTGG;> TTTTTTTTTGCTCACTGCCCGCTTTCGAGAGCCAG;> AAATTGTCCACAAGTGAAGGCTGTCCTACCGTAAA;> TTTTTTTTTAGCCGGAAGCATAAAGTGAGGATTTA;> TCCTTTGATTATCATGGAAAGTTGAGTATACTGCT;> GATGATGATCAGTGGGCCTATGCAATTAAAAATTA;> AGGAACACTGCACAATTTTCAGGTTTCTTGGATGA;> TTTTTTTTTTCGTAATCATGGTCATAATCCTGATT;> CTTGGGTAGTGGCTCACAAGGGATGTTCCAGGAAC;> TAACACCCTGACGCAGTGGTCATGGTAAGGAACGT;> GAACCTACCGTATACATTAAATAATATTCACAAAC;> GCTAGTCGCAGGATCTTCAATAACCCCCGATTTAG;> GTGAGTGCAAAATTTAAATCATGTGGCCTGCATAG;> AGGTTATGGAGTGTTTTTGCTCTCTGTAGCGAGAA;> GATGAGTCCTCTTGTTGAGTTGCCTGAGCCTTACC;> TGCTTCTGTAAATCAGCAAAATTAGTACAGAGGCT;> CCCATATGCCCTAGAAACAAAGTGACCATGAGGGA;> CTTAATTTTCCCTTAGAATAGTACCGCCACCCTCA;> ATCATAGGTCTGAGGTTATATCTGAGTTATTCCAC;> TAGATTAAGACGCTAGACAAATTCAGGGTTTGTCG;> AATCGCAGAGAAGAGATGCACCCCCTTGAAAACAT;> AATAAGGCGTTAAAAAAAGCCAAGGAATCCAAAAA;> TGAAATACCGACCGTGCGTTAGAGAATAGAGCCTT;> GCCACAAGTAATAAGAGAATACCAGACGAGAAGAG;> TTTTTTTTTATGGGGTGGTGGAGCTCTGCTGACCT;> TTTTTTTTTGTGATGACTCTGATGGTCAAAGCAGA;> TGGAGGAGAGATTTCCTCCCAATGATTCGCCCAGT;> AGCCCTATGCATATACCAATCTAGCAAGTATGGTC;> CAAATCAGATATAGACGAGCAAGGACTAGCCGACA;> AACTATGTCAATTAATTGCAGGCGGGAGAAACAGC;> TTTTTTTTTCTTATTAGTTGCTTAAGCCACCTGTT;> AGGTTGCATTGACTCCACATACAATATACCATAGT;> GCAGCCTCTACCTATTGTAGGTTTATTAGAAGATG;> TTTTTTTTTGGCGATTAAGTTGGGTAATCCAAATA;> ATTAAGTGCATTAGGGAGAGTAATCTTACCAACGC;> GTCAAAAAGTTAAGGACGGTCCAAAGCTGCTTTTT;> TCTGAGTGAGCTCCGACTCTTTCATTAGAAATTCA;> GATGTTTATATCAGGAGAGAATTACTCTTTACTAG;> GAGCATGAGAATTGATGAAAATGCGATTTTTTGTT;> TTTTTTTTTTTGGGAAGGGCGATCGGCAATAATAA;> TGCCCACCTACACAATAAATCAAAAGAATTGGAAC;> CGCAATACATTTTATTAGGAACGCCAAAGACAAAA;> TAGGAATGACTGATTGTGTAACAGACTTGGAAAGC;> TCATAGGAATGCTCTGGAATTTTGACTATTCACCA;> TTGCGACAGAATCATCCATGAAAAGATCAAATCAA;> TTAACAGGCCCTAGTAGAAGGGATTGCAGCCAGGA;> TAGCTGTTTCCTGTGTGAATTTTTTTTT;> GGGGATAAGAAATATACCTTTAGCTGGC;> GAATATACCGAGCTCGAATTTTTTTTTT;> CAGATGAGTCTTGGAGGAGAAATTTCAT;> CAATAACGGCAAGATGAGGGTATGAAAC;> ATACCACCTCGATAAAGACTTTTTTTTT;> GCACCGGCTATGTTGGACCTTTGGCAGA;> TTCATACAGGGCTTAAGCTTTTTTTTTT;> TTGAACAACGCCGTCGAGAGGTAGAACA;> AGCGACATTTCACATAAATTTTTTTTTT;> GAGACTCAGGATAATGCCCAGGGATTCGCCTGATT;> AAAATCTTGCGAATGTGGAATACCTTATCTGTAGC;> TCTTAATATAGGATAGCTAATGCAGAACTAATTTA;> AAGGCCGCTACTGGGAAGCTATAAAGTAATTCTGT;> ATGACAACTTGATAACAAGAATTTATCAACAATAG;> CGATTATATTTTATAAGCCCCACTTGCATTGAGGA;> TCTGAATAAAGTACGCTATTTTCTCTCAGTGTTTG;> TCTAAGCTGAATAGCTACCTCAGTATTTTTTTTTT;> CTTGAAAATAGACAACAGATTGGCATGGAGACCAC;> GAATACAAACGTAAAATCATATGGCCGGAACGAGG;> AAAAATCATTTCAGGCTGCGCAACTGTTTTTTTTT;> TCCACAATAAAGTCAAGAGTAATGAACGTTTGCTG;> GTGCATGGATACCTCCTCTAGACAACCCAGGTAGC;> GCTGTACCAATTATTTTGTACTGGCTTTTTTTTTT;> TTTTTTTTTTACCCAGTCAATAGTAAAAGTCCTAA;> CATGCCTTGCTACTTTGACCCGGATATAATACCAG;> ATACTCTAAAAATACAGACCTTTGAAAGAGCGCTA;> TGTGTATATGTTGGTAATCACTTCTTTTTTTTTTT;> TAAACCATGTAGCAAGGTGCTTGCGGGAGTACCGC;> GGCCACATTTAAGACCCAGCAATTGGTTTTTTTTT;> TTTTTTTTTATTGGTGTGGTTTGTGTTTAATAAGT;> GATAAGAGGTCACCACAACGCGGTTGCTAAGTCAG;> GCTTAATTAATTGCAGACAGCATTTGAGGTTCTCA;> CTACAGGATTTAGTTTTCTGGAGGGGGTCTGTACT;> TTGGGGTCAAAGGGTAAATCAATGTGCGTTTTATC;> AAAGAACGATAGGGAATCAATAAGGTAGAAGGATG;> TAATGATAACTCGATATTTTAGGCAAAATGACAGG;> ACCTTCTTAAGTAGGTATTGTATTCTAGCAACCGA;> CAATGCAAGAGAGGTGAGTAGGCCTAGGAAACTGC;> AGGTGAAACCACGGGTGAGAAACACCAGAACGA;> ACTGTGCACCTATGAGGAAGAGGGGTTCCCAT;> TTTTTTTTTTCTGCTGTCCTTATCATAAGTAA;> AAGAGTCCACTATTATCCCTTCTGGAAA;> TCACCTGCCCTTCACCGCCTTTTTTTTT;> CTATGTTCACCAGTGAGACTTTTTTTTT;> TAGACAGCGCTAGGGCGCTGGTTGACGG;> TTTTTTTTTGGGTGGTTTTTCTTGTTGC;> GTAAAAGGGGATTTGCAAGGGCGACATT;> GTCACACCATGGAATTTATCTATCACCA;> GGGACATCATTGCATTAAGCCACAAGTC;> TGGCACGGCCAACGCGCGGTTTTTTTTT;> ATGCGCGCGTTTTCCGGAAACAAAGTAG;> GGGAAACCTGTCGTGCCAGTTTTTTTTT;> AACACATTAATTGCGTTGCTTTTTTTTT;> CATTTGGACTAGCCTATGATGAAAAGGT;> CAGTTGAAAGGACTGGATCTGCTAGTAC;> TATCTAAGCCAAGCTACTGTGTAATGTG;> TTGTAAAGCCTGGGGTGCCTTTTTTTTT;> CTTAGGGCATTATGCAAGGGCGCCCCTA;> AAATTCCACACAACATACGTTTTTTTTT;> ACCTACTCAGGTGTGGCTTAAGAAACTT;> GGAATTATTACCGTAGTTTTAATCACAA;> TGACTATAGGCCCCCATGAAAGCATAAC;> GCGATTAAGAGGAATATCCTAATCCACC;> AGCGATGTTTAGCTATATTTTTTTTTTT;> TTTTTTTTTAATGGTCAATAACCACCAG;> CCATTAGATACATTTCGCATTTTTTTTT;> GTCAGGATAACGATATCATGTAACTGTT;> CCGCGCTTAATGGAGCAGATGCTTTTAA;> AGCCGGCTGCGCGTACTGTCCATACAGT;> TCTTGTCATGGTTTCGCCAAATTGAGTG;> GCCAGGCGTCACCAGCCACCAATATTAC;> GATGAGTCTGGAGTCAGCATTTTTTTTT;> AGTAATCCTGGAGAAGTAATTTTTTTTT;> CGACTTTTTCAAATATTATTAAGGAGTC;> TCTTACCAATGGTTCCTGCTGCTTGGAT;> CTCTGGTTATCACAGCAAGTTTTTTTTT;> TCCCCATAGGAGTTACATCAACATGTAC;> TTATTTAACAACGCCAACATGGCGCCTG;> AATACTTCACCCTATATAGTTTTTTTTT;> AAGACCTATCTTAATAGTACTACCCCAG;> GTCCTGACCGATAGATTGAATTTCTTAA;> ATTCCAATAGGTTGTGTGGTTTTTTTTT;> AGCTGGAAGATTGAGAGGCTTTTTTTTT;> AACGCGAGGCGTTTCTTATCCAACGGGT;> AATGGACACCCCACATGGTTTTTTTTTT;> TAAGGGGGATGTGCTGCAATTTTTTTTT;> TTTTTTTTTTTACGCCAGCTGGCGAAAC;> CCTGCGGGCCTCTTCGCTATTTTTTTTT;> CTGGCTGCAGTTGTAGGTTGGCAACTCT;> ACCTTTAAAGGTTGTACTGAACACCCTG;> AGGTTTGGTTACCAGAAGGAAACCGAGA;> GTAAGCAGATAGCCAAAAGAACCAGTGC;> CTGTAAAGAAGGCATGGGCACTGTCACT;> CTAAACGCAAAGACTTATCACCGTCAAC;> TAAGGGCGCTGAGCATACCTACCACCGA;> TTTTTTTTTGCGGATTGACCGTAATGCC;> CAGGACACAAGGATTTAATACGTATGGA;> CTAAATGCCTCCCTCACTAACACATGGC;> TACTCCGTGGGAACAAACGTTTTTTTTT;> TTTTTTTTTTAACAACCCGTCGGATTAT;> TTTTTTTTTTAGCCAGCTTTCATCAAGA;> AACGCGTCTGGCCTTCCTGTTTTTTTTT;> TTTTTTTTTCGCCATCAAAAATAATTAT;> GAATTTCAAGGCAGTGGGTATTGAATGG;> GCCTAAGACCAGCAAGGGTTTCAACACC;> AGTGTTCGTTGATATTTAACATTGGTCT;> CATGCATAATAGGTAAGAAAAGACAGCT;> GAGCCAGATTGTATAAGCATTTTTTTTT;> TTTTTTTTTTGTGTGATGGGGAAAGACT;> ATCGGTTAGTTTCAGTTGGCTTGAATTT;> TTTTTTTTTGATTGAAGTGATTCTCTCT;> ACAGGAGTTGAAAGCATTATTTTTTTTT;> TTTTTTTTTAACAAGCCTACTAGCAGAT;> TTTTTTTTTTTATAACATTCCAAGTTAA;> TTTTTTTTTTAGACTGGAGGTGTGTACT;> CCATGTTACTTAGGCGAAATCCCGACTT;> TTTTTTTTTAAAGATTCAAAAGGGTGCT;> CGCTGAGTAATGTGTAGGTTTTTTTTTT;> GACCAGGCGCATCACTAGTCCTATCAAT;> TTTTTTTTTTATTTTAAATGCAATGCCA;> ATGGGTCTGCAAGATTGAGATATCATAA;> TGAAAGTGGGTATATCAAGTTTTTTTTT;> AAGAAGTACCTGGAGTGTACAAACAAAG;> TAACCCAGTGATAATAGCTGCGCAGAGA;> GGTGAACATTTTAAGAGCATTGCCTCTG;> TTTTTTTTTCATTTCTCCGAA;> TGTTTAGGAAAAGACTTGAAG;> AGTATAATTTCAACTATCAGC;> TTTTTTTTTTCAGGATTTATG;> CCGGAAACCAGGTTTTTTTTT;> GTGTGGCAACATATAAAAGCC;> AGCCAGCTTTCCTTTTTTTTT;> TTTTTTTTTAGGAAGATCGCA;> AGTATCGGCCTCTTTTTTTTT;> AAGGAATTAGAGCCAGCAAGT;> GCATCTGCCAGTTTTTTTTTT;> CTTTAGCCATCGATGTGCAGT;> TTGGTGTAGATGTTTTTTTTT;> AATTATTGGCAATGTATTAAA;> TAGGATTTTTAATCGGGGTAC;> TTTTTTTTTTTTAGGGGAGGT;> TTGCTTTCGAGGTGGATTGCT;> TGCCACTTCCATTAGGTATTC;> TTGGGCTTGAGATGGTTTA>[4x]LTEQPNWLMQRAQLTPERIALIYEDQTVTFAELFAASKRMAEQLAAHSVRKGDTAAILLQNRAEMVYAVHACFLLGVKAVLLNTKLSTHERLFQLEDSGSGFLLTDSSFEKKEYEHIVQTIDVDELMKEAAEEIEIEAYMQMDATATLMYTSGTTGKPKGVQQTFGNHYFSAVSSALNLGITEQDRWLIALPLFHISGLSALFKSVIYGMTVVLHQRFSVS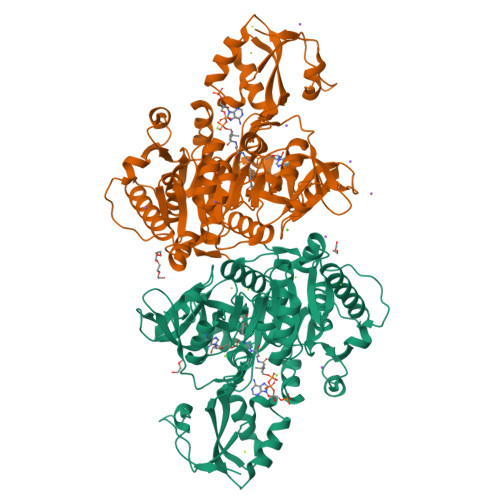DVLHSINRHEVTMISAVQTMLASLLEETNRCPESIRCILLGGGPAPLPLLEECREKGFPVFQSYGMTETCSQIVTLSPEFSMEKLGSAGKPLFSCEIKIERDGQVCEPYEHGEIMVKGPNVMKSYFNRESANEASFQNGWLKTGDLGYLDNEGFLYVLDRRSDLIISGGENIYPAEVESVLLSHPAVAEAGVSGAEDKKWGKVPHAYLVLHKPVSAGELTDYCKERLAKYKRPKKFFVLDRLPRNASNKLLRNQLKDARKGELL>[2x]MNISTIVSNLKDLILEVRAPYDLEITGVSNHSSKVKKGDLFICRRGEKFDSHEI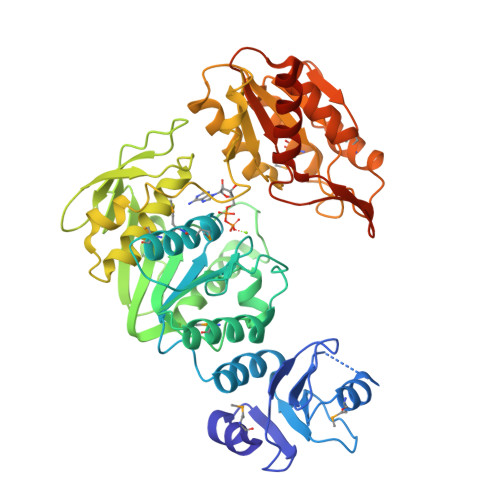IPEVMEKGAVAVVVEREIDLDFPYIQVFDSRYFEAKVASLFFEDPWKDVLTFGVTGTNGKTTTTMMIYHMLTSLGERGSVLTTAVKRILGNSYYDDITTPDAITILSAMKENREGGGKFFALEVSSHALVQQRVEGVRFDVGIFTNISRDHLDFHGTFENYLKAKLHLFDLLKDDGVAVLNESLADAFNRKSRKITFGTSKNADYRLGNIEVSWEGTQFVLETPDGLLKVFTRAIGDFNAYNAAAAIAALHQLGYDPKDLASSLETFTGVEGRFEVVRGAKKIGLNVVVDFAHSPDALEKLLKNVRKISQGRVIVVFGAGGNSDRGKRPMMSEVASKLADVVILTTDDPRGEDPEQIMEDLIKGIDKRKPYLVLFDRREAIETALTIANRGDSVVIAGRGHERYQIIDEEKKVPFQDREVVEEIIRDKLKGRKYAQLEHHHHHH>TEKFDFGTMVQWAYDHKYAEESKIAYEYALAAGSDSNARAFLATNSQAKHVKDCATMVRHYLRAETQALSMPAYIKARCKLATGEGSWKSILTFFNYQNIELITFINALKLWLKGIPKKNCLAFIGPPNTGKSMLCNSLIHFLGGSVLSFANHKSHFWLASLADTRAALVDDATHACWRYFDTYLRNALDGYPVSIDRKHKAAVQIKAPPLLVTSNIDVQAEDRYLYLHSRVQTFRFEQPCTDESGEQPFNITDADWKSFFVRLWGRLDLIDEEEDSEEDGDSMRTFTCSARNTNAVD[6x];>GSRATVFKLGLFKSLFLCSFHDITRLFKNDKTTNQQWVLAVFGLAEVFFEASFELLKKQCSFLQMQKRSHEGGTCAVYLICFNTAKSRETVRNLMANMLNVREECLMLQPPKIRGLSAALFWFKSSLSPATLKHGALPEWIRAQTTLNAAAA[2x]

Helicases use the energy of nucleoside triphosphate (NTP) hydrolysis to translocate and unwind DNA, providing the single-stranded template (ssDNA) for accurate copying by DNA polymerase. A hexamer of the C-terminal helicase domain (E1HD) can function alone to unwind dsDNA in vitro. The E1HD subunit can be sub-divided into the collar domain and the NTPase motor domain that form rings in the E1HD structure.

Here we present a near-atomic resolution (3.9 Å) cryo-EM structure of E1 revealing clearly all arms of the RF and the dsDNA unwinding point for an AAA+ hexameric helicase. The structure demonstrates unambiguously the positions of the dsDNA, the 3′ssDNA active strand within the entire central channel of the E1HD and the 5′ssDNA passive strand, positioned on the top of the collar ring. The dsDNA separation point, the RFJ, is located at the entrance to the collar tunnel. In the E1 helicase, dsDNA is separated at the entrance to the collar domain ring, as the AAA+ motor pulls one ssDNA strand through the complex and the RFJ against the collar ring. The OBD of subunit B interacts with the dsDNA while the OBD from subunit E interacts with the 5′ passive ssDNA strand and is located close to the side of the E1HD collar ring. While the dsDNA sequence of the fork does not contain an E1BS-like sequence, the cryo-EM structure indicates that OBD B interacts with the dsDNA via an interaction between the DBL and the major groove at the sequence TGTGA in the passive DNA strand, 16-20 nucleotides from the RFJ. In the E1RF cryo-EM structure, the 5′ ssDNA is diverted from the separation point at an angle of 95° relative to the dsDNA axis, passing in a groove between E1 subunits D and E. Second, the 5′ ssDNA is trapped in a groove between collar subunits D and E where the TNS loop of subunit D and Lys310 in the inter-domain linker of subunit E escort the unwound 5′ ssDNA from the complex. In the E1RF complex, as in E1HD/ssDNA/ADP, six nucleotides of the 3′ ssDNA strand form a right-hand helix with the β-hairpins of the AAA+ domains, before it exits from the channel. The β-hairpin of subunit B does not contact the 3′ ssDNA either, since its His507 is turned away from ssDNA compared to the crystal structure. Our observations, therefore, appear to be consistent with the coordinated escort mechanism for ssDNA translocation, although a different conformational state appears to be captured in the cryo-EM structure, where the subunit A β-hairpin has disengaged from ssDNA and has not yet migrated back to the top of the complex to re-engage with ssDNA.> ETGSLYLWIDAHQARVLIGFEEDILIVSEGKMAPFTHDFRKAQQRMPAIPVNIHSMNFTWQAAGQAEYFYEFLSLRSL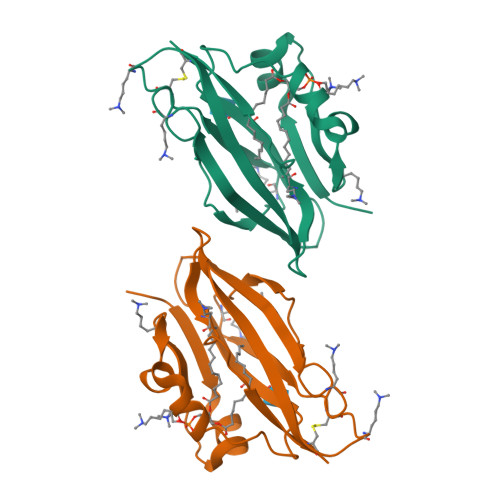DKGIMADPTVNVPLLGTVPHKASVVQVGFPCLGKQDGVAAFEVDVIVMNSEGNTILKTPQNAIFFKTCQGTKHHHHHH morpholine | C4 H9 N O | 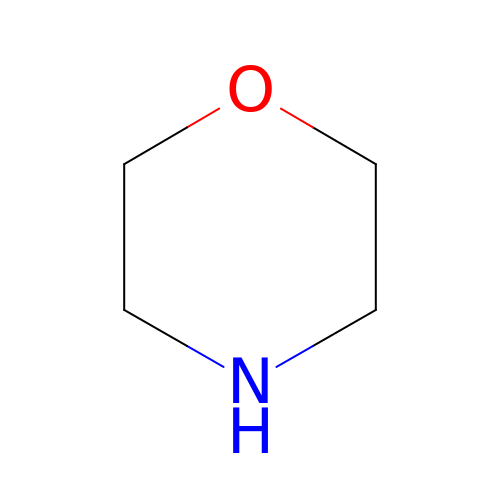YNAVUWVOSKDBBP-UHFFFAOYSA-N>YQLQPLSLDSVPWRRQPGQQVLWIGCSDSGCDELESSGLPADEIFEYRSLGNMMVDDLSCKATLGYALDSLKIRNIVICGHYGCHIASGEVNAGLQKPWSSVLDTLRSTHRRTLDSLTGTERDRALVELNVLEQVHSLRQSAEAAEALQKQQ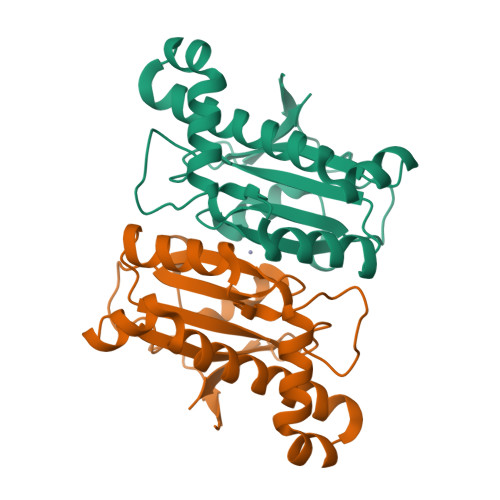LNIWGMVYDKATKRGYQLI[2x]> METLSFEFPAGQPGRGRALVGCVGSGDLEVLLEPGQPGKLSIQVQTSVNGSASRWQHLFERLFDGQTPP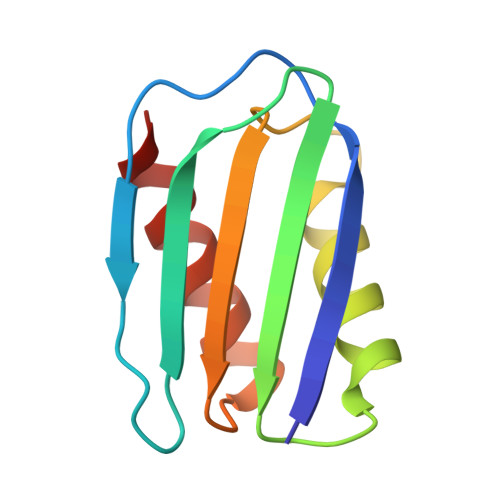ALLIDIHDFGATPGVVRLRLEQGFEEIGHD N,N'-(butane-1,4-diyl)bis{2-[2,3-dichloro-4-(2-methylidenebutanoyl)phenoxy]acetamide} | C30 H32 Cl4 N2 O6 | 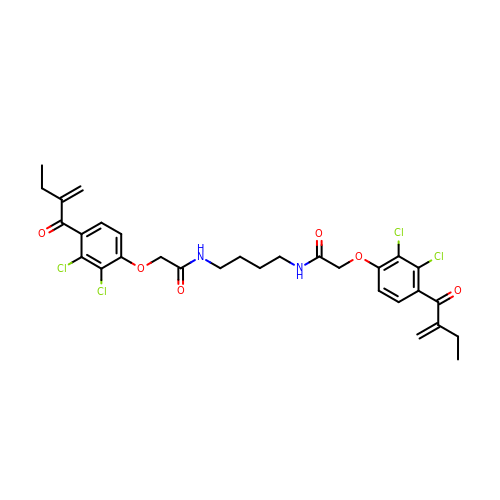DJUYDJABFNZJNL-UHFFFAOYSA-N> GSPCVEVVPNITYQCEELNFYKIPDNLPFSTKNLDLSFNPLRHLGSYSFFSFPELQVLDLSRCEIQTIEDGAYQSLSHLSTLILTGNPIQSLALGAFSGLSSLQKLVAVETNLASLENFPIGHLKTLKELNVAHNLIQSFKLPEYFSNLTNLEHLDLSSNKIQSIYCTDLRVLHQMPLLNLSLDLSLNPMNFIQPGAFKEIRLKELALDTNQLKSVPDGIFDRLTSLQKIWLHTNPWDCSCPRIDYLSRWLNKNSQKEQGSAKCSGSGKPVRSIICPT

Toll-like receptor 4 (TLR4), a superfamily of LRR proteins, is the principal receptor mediating innate immune responses against infections by Gram-negative bacteria. In this process, myeloid differentiation protein 2 (MD2) recognizes various lipopolysaccharides (LPSs) released from the Gram-negative bacteria, forming a complex with LPS at its hydrophobic pocket. In an attempt to prevent the systemic immune response caused by LPS, a TLR4 decoy receptor was constructed by combining LRR modules from the TLR4 ectodomain and VLR. The constructed decoy receptor was shown to attenuate the TLR4-mediated signaling process by trapping MD2, implicating a potential therapeutics for bacteria-induced sepsis and inflammation.

We reasoned that substituting these residues for charged residues would increase the interaction with MD2 via charge interactions. It is likely that the M41E and S62E mutations would induce strong interactions with positively charged Arg-68 and Lys-109 of MD2. To analyze the interaction interfaces of other single mutants (M41E and V134L), we obtained the modeled interaction interfaces by superimposing their apo structures into the complex structure of the wild-type decoy receptor/MD2. For this, we determined the crystal structures of the single mutants in free form at a −2.4 Å resolution. The M41E mutant was designed to have a strong charge interaction with a positively charged Lys-109 in MD2 and the substituting Glu-41 was shown to be able to form an additional interaction with Lys-109 of MD2, resulting in a significant increase in binding affinity. However, the M41E mutant exhibited an increase of 86.31 kJ/mol in the Coulomb interaction and a decrease of the LJ potential by 4.53 kJ/mol, respectively. Thus, an increase in the binding affinity of the M41E mutant was likely to come mainly from the increased charge interaction. Superposition of the mutants on the wild-type revealed that their original backbone structures were retained, which represents the structural characteristics of repeat proteins.>[4x]MELFLAGRRVLV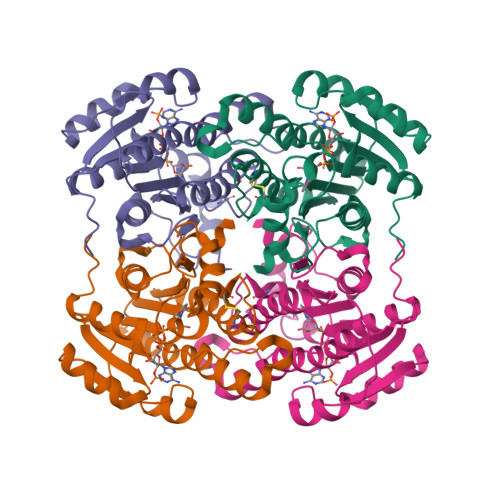TGAGKGIGRGTVQALHATGARVVAVSRTQADLDSLVRECPGIEPVCVDLGDWEATERALGSVGPVDLLVNNAAVALLQPFLEVTKEAFDRSFEVNLRAVIQVSQIVARGLIARGVPGAIVNVSSQCSQRAVTNHSVYCSTKGALDMLTKVMALELGPHKIRVNAVNPTVVMTSMGQATWSDPHKAKTMLNRIPLGKFAEVEHVVNAILFLLSDRSGMTTGSTLPVEGGFWAC>[6x]MM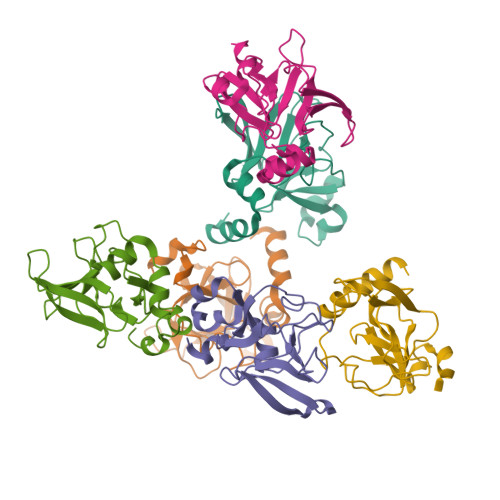AYNKEEKIKSLNRMQYEVTQNNGTEPPFQNEYWDHKEEGLYVDIVSGKPLFTSKDKFDSQCGWPSFTKPIEEEVEEKLDTSHGMIRTEVRSRTADSHLGHVFNDGPGPNGLRYCINSAALRFVPKHKLKEEGYESYLHLFNK>MDILIVNPDDFEKGVEEVKELKRHGAKIIAYISKSAEELKKAEKAGADILIVNPDDFEKGVEEVKELKRHGAKIIAYISKSAEELKKAEKAGADILIVNPDDFEKGVEEVKELKRH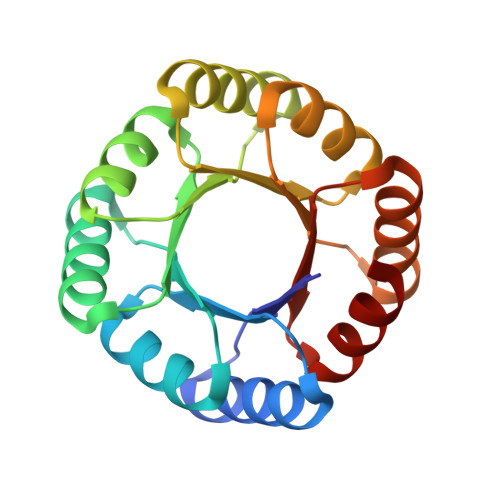GAKIIAYISKSAEELKKAEKAGADILIVNPDDFEKGVEEVKELKRHGAKIIAYISKSAEELKKAEKAG[4x]V/A-ATPase is a motor protein that shares a common rotary catalytic mechanism with FoF1 ATP synthase. The V1 domain of Tth V/A-ATPase (A3B3D1F1) is an ATP-driven rotary motor where the central DF shaft rotates inside the hexameric A3B3 containing three catalytic sites, each composed of an AB dimer. When powered by ATP hydrolysis, the V1 domain rotates the central rotor against the A3B3 hexamer, composed of three catalytic AB dimers adopting different conformations (ABopen, ABsemi, and ABclosed). Here, we report the atomic models of 18 catalytic intermediates of the V1 domain of V/A-ATPase under different reaction conditions, determined by single particle cryo-EM.

The nucleotide-free V/A-ATPase (Nucfree) was used for cryo-grid preparation under different ATPase reaction conditions. We obtained structures of three rotational states of V/A-ATPase without nucleotide; state1 at 3.1 Å, state 2 at 4.7 Å, and state 3 at 6.3 Å resolution, with the DF shaft positions differing by 120° in each case. Using signal subtraction of the Vo domain, we achieved resolution of 3.0 and 4.1 Å for the V1 domain including half of the EG stalk in state1 and 2, allowing us to build atomic models of the V1 domain of these states. We identified a cryoEM structure of the original state1 from 39,902 particles at 3.1 Å resolution and another substate from 24,101 particles at 3.1 Å resolution. In the ABclosed and ABsemi dimers, densities for the catalytic side chains are well resolved, but no density corresponding to nucleotide was observed. Hereafter we refer to the structure as the Vnucfree. The structure of Vnucfree is very similar to the previously reported ADP inhibited structure. In addition, the Vnucfree is also similar to the structures under the saturated-ATP condition determined in this study, with the positions of the catalytic side chains almost identical in both cases. The Vnucfree in the ground state is activated by the binding of ATP to the catalytic sites.

>[3x]MIQGVIQKIAGPAVIAKGMLGARMYDICKVGEEGLVGEIIRLDGDTAFVQVYEDTSGLKVGEPVVSTGLPLAVELGPGMLNGIYDGIQRPLERIREKTGIYITRGVVVHALDREKKWAWTPMVKPGDEVRGGMVLGTVPEFGFTHKILVPPDVRGRVKEVKPAGEYTVEEPVVVLEDGTELKMYHTWPVRRARPVQRKLDPNTPFLTGMRILDVLFPVAMGGTAAIPGPFGAGKSVTQQSLAKWSNADVVVYVGCGERGNEMTDVLVEFPELTDPKTGGPLMHRTVLIANTSNMPVAAREASIYVGVTIAEYFRDQGFSVALMADSTSRWAEALREISSRLEEMPAEEGYPPYLAARLAAFYERAGKVITLGGEEGAVTIVGAVSPPGGDMSEPVTQSTLRIVGAFWRLDASLAFRRHFPAINWNGSYSLFTSALDPWYRENVAEDYPELRDAISELLQREAGLQEIVQLVGPDALQDAERLVIEVGRIIREDFLQQNAYHEVDAYCSMKKAYGIMKMILAFYKEAEAAIKRGVSIDEILQLPVLERIGRARYVSEEEFPAYFEEAMKEIQGAFKALA;>MDLLKKEYTGITYISGPLLFVENAKDLAYGAIVDIKDGTGRVRGGQVIEVSEEYAVIQVFEETTGLDLATTSVSLVEDVARLGVSKEMLGRRFNGIGKPIDGLPPITPEKRLPITGLPLNPVARRKPEQFIQTGISTIDVMNTLVRGQKLPIFSGSGLPANEIAAQIARQATVRPDLSGEGEKEEPFAVVFAAMGITQRELSYFIQEFERTGALSRSVLFLNKADDPTIERILTPRMALTVAEYLAFEHDYHVLVILTDMTNYCEALREIGAAREEIPGRRGYPGYMYTDLATIYERAGVVEGKKGSVTQIPILSMPDDDRTHPIPDLTGYITEGQIQLSRELHRKGIYPPIDPLPSLSRLMNNGVGKGKTREDHKQVSDQLYSAYANGVDIRKLVAIIGEDALTENDRRYLQFADAFERFFINQGQQNRSIEESLQIAWALLSMLPQGELKRISKDHIGKYYGQKLEEIWGAPQALD[3x];> MSQVSPTRMNLLQRRGQLRLAQKGVDLLKKKRDALVAEFFGLVREAMEARKALDQAAKEAYAALLLAQAFDGPEVVAGAALGVPPLEGVEAEVENVWGSKVPRLKATFPDGALLSPVGTPAYTLEASRAFRRYAEALIRVANTETRLKKIGEEIKKTTRRVNALEQVVIPGIRAQIRFIQQVLEQREREDTFRLKRIKGKIEAREAEEEGGRPNPQVEIGAGL;> MAVIADPETAQGFRLAGLEGYGASSAEEAQSLLETLVERGGYALVAVDEALLPDPERAVERLMRGRDLPVLLPIAGLKEAFQGHDVEGYMRELVRKTIGFDIKL;>MTGGLVLNAISRAGGAMGGLGLIKSLAEKEKQLLERLEAAKKEAEERVKRAEAEAKALLEEAEAKAKALEAQYRERERAETEALLARYRERAEAEAKAVREKAMARLDEAVALVLKEVLP[2x];>MSKLEAILSQEVEAEIQALLQEAEAKAEAVKREAEEKAKALLQARERALEAQYRAALRRAESAGELLVATARTQARGEVLEEVRRRVREALEALPQKPEWPEVVRKLALEALEALPGAKALVANPEDLPHLEALARERGVELQAEPALRLGVRAVGAEGKTQVENSLLARLDRAWDALSSKVAQALWG[2x]>RRSPPADAIPKSKKVKVSHRSHSTEPGLVLTLGQGDVGQLGLGENVMERKKPALVSIPEDVVQAEAGGMHTVCLSKSGQVYSFGCNDEGALGRDTSVEGSEMVPGKVELQEKVVQVSAGDSHTAALTDDGRVFLWGSFRDNNGVIGLLEPMKKSMVPVQVQLDVPVVKVASGNDHLVMLTADGDLYTLGCGEQGQLGRVPELFANRGGRQGLERLLVPKCVMLKSRGSRGHVRFQDAFCGAYFTFAISHEGHVYGFGLSNYHQLGTPGTESCFIPQNLTSFKNSTKSWVGFSGGQHHTVCMDSEGKAYSLGRAEYGRLGLGEGAEEKSIPTLISRLPAVSSVACGASVGYAVTKDGRVFAWGMGTNYQLGTGQDEDAWSPVEMMGKQLENRVVLSVSSGGQHTVLLVKDKEQ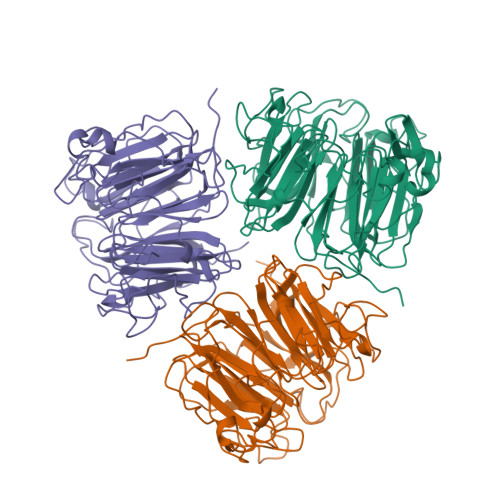S[3x]> MTTVKLTYFGHSAFHVEVDGVGIAIDPWITNPLSKTTLEDYLKNFKTDLVVITHAHEDHIGDALEIMRRTGAKFFSIHEIYVDLTQKGFQGIGANI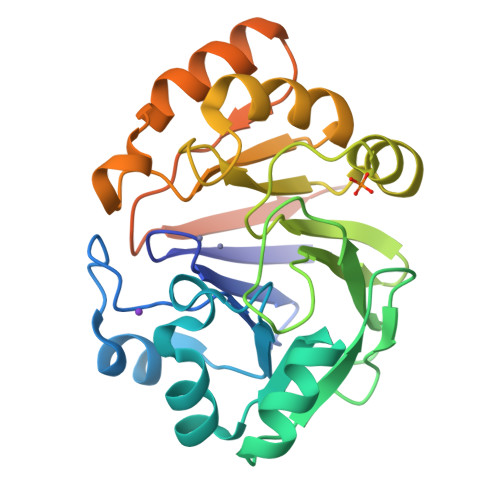GGPAKLDDVAPGLGIALTPATHSSYDKGVPTGAIIFKDGKALVYHAGDTGLFAEMQFIGELYAPKVALLPIGGHYTMDIEQALLATKLLRPEVVVPMHYNTFPPIRADPNEFKQKVESAGLAKVRVMEPGETVTFEFKGRQLGPEQKLISEEDLNSAVDHHHHHH> MIIDLSQLPEPEVIENLDFETIYQELLGDFREAMAGEWTAEVESDPVLKLLQLAAYRELLLRARINDAARAVMLAYASGADLDQIGAGFNVQ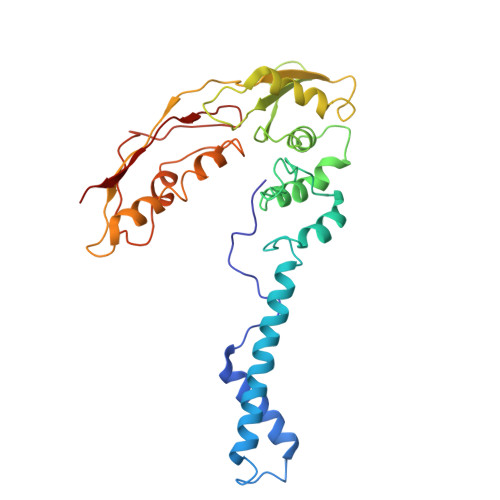RLLIRPAQPEAVPPVEAQYESDKSLRNRIQLAFEQLSVAGPRNAYIAHALGADGRVADASATSPAPCEVLISVLGVEGNGQAPEAVLQAVRLALNAEDVRPVADRVTVRSAGIVPYQVKAQLYLFPGPEAELIRAAAEASLRDYISAQRRLGRDIRRSALFATLHVEGVQRVELQEPAADVVLDETQAAYCTGYAITLGGVDE> SQINQVRPKLPLLKILHAAGAQGEMFTVKEVMHYLGQYIMVKQLYDQQEQHMVYCGGDLLGELLGRQSFSVKDPS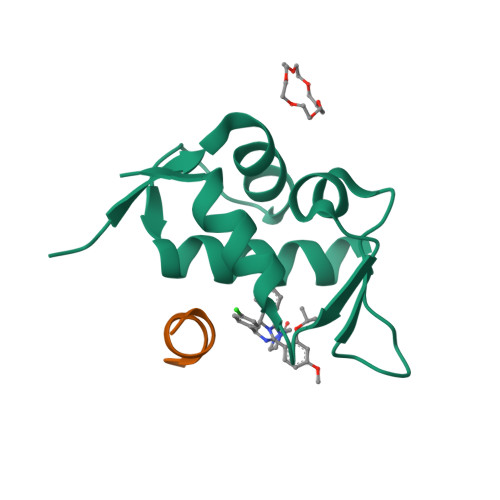PLYDMLRKNLVTLAT;> DLENLYFQG>[3x]XRMKQIEDKIEEIESKQKKIENEIARIKKLLQLTVWGIKQLQARILX;>[3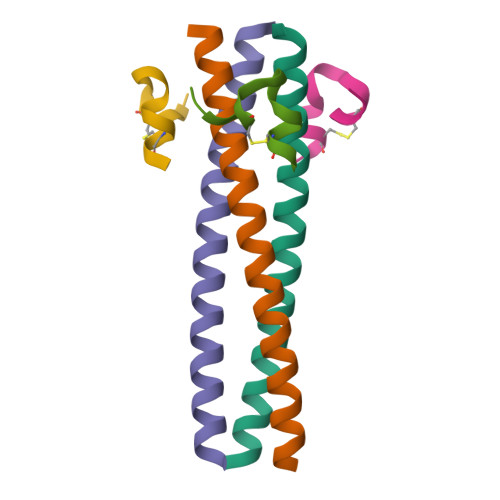x]XKGHPCDYPEWQWLCELX>[2x]MDDDDKMDNECTTKIKPRIVGGTASVRGEWPWQVTLHTTSPTQRHLCGGSIIGNQWILTAAHCFYGVESPKILRVYSGILNQSEIKEDTSFFGVQEIIIHDQYKMAESGYDIALLKLETTVGYGDSQRPICLPSKGDRNVIYTDCWVTGWGYRKLRDKIQNTLQKAKIPLVTNEECQKRYRGHKITHKMICAGYREGGKDACKGDSGGPLSCKHNE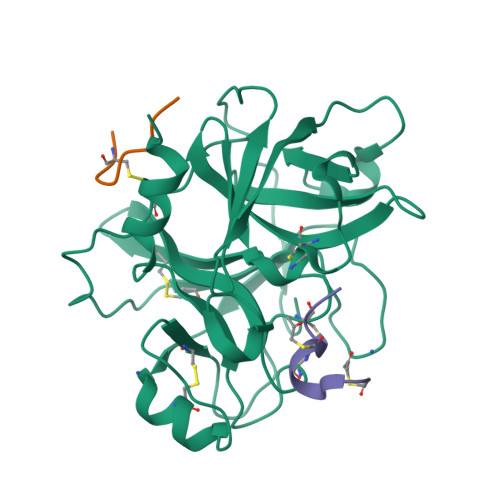VWHLVGITSWGEGCAQRERPGVYTNVVEYVDWILEKTQAVHHHHHH;> CVNIMCCRCPX3-(3,4-dichlorophenyl)sulfanyl-1$l^{4},2,7,8-tetrazabicyclo[4.3.0]nona-1(6),2,4,7-tetraen-9-one 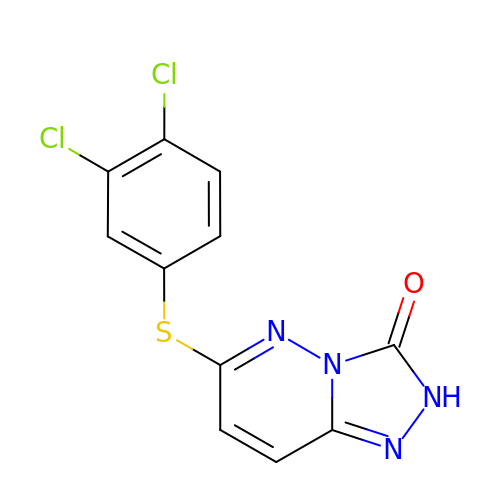| C11 H6 Cl2 N4 O S | DYBIDXYUMDMCON-UHFFFAOYSA-N> VSLEQALKILKVAAELGTTVEEAVKRALKLKTKLGVSLEQALKILEVAAELGTTVEEAVKRALKLKTKLGVSLEQALKILEVAAKLGTTVEEAVKRALKLKTKLGVSLEQALKILKVAAELGTTVEEAVKRALKLKTKLGVSLEQAL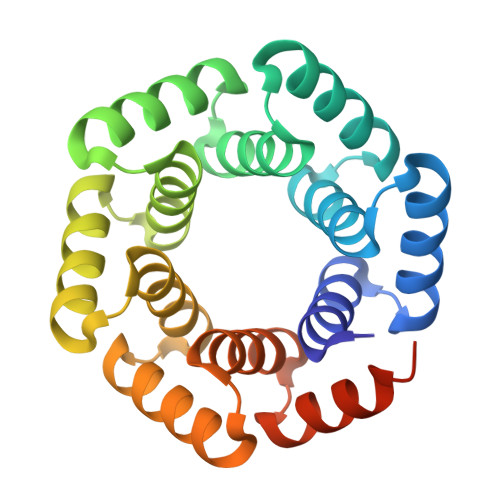KILEVAAELGTTVEEAVKRALKLKTKLGVSLEQALKILEVAAKLGTTVEEAVKRALKLKTKLGGWLEHHHHHH>ETGFPEDSEPISISHGNYTKQYPVFVGHKPGRNTTQRHRLDIQMIMIMNGTLYIAARDHIYTVDIDTSHTEEIYCSKKLTWKSRQADVDTCRMKGKHKDECHNFIKVL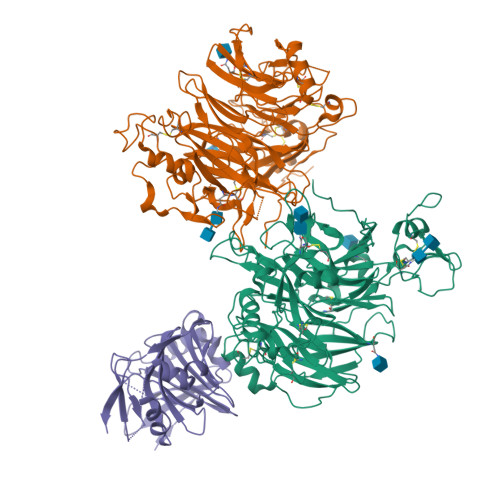LKKNDDALFVCGTNAFNPSCRNYKMDTLEPFGDEFSGMARCPYDAKHANVALFADGKLYSATVTDFLAIDAVIYRSLGESPTLRTVKHDSKWLKEPYFVQAVDYGDYIYFFFREIAVEYNTMGKVVFPRVAQVCKNDMGGSQRVLEKQWTSFLKARLNCSVPGDSHFYFNILQAVTDVIRINGRDVVLATFSTPYNSIPGSAVCAYDMLDIASVFTGRFKEQKSPDSTWTPVPDERVPKPRPGCCAGSSSLERYATSNEFPDDTLNFIKTHPLMDEAVPSIFNRPWFLRTMVRYRLTKIAVDTAAGPYQNHTVVFLGSEKGIILKFLARIGNSGFLNDSLFLEEMSVYNSEKCSYDGVEDKRIMGMQLDRASSSLYVAFSTCVIKVPLGRCERYGKCKKTCIASRDPYCGWIKEGGACSHLSPNSRLTFEQDIERGNTDGLGDCHNGSWSHPQFEK[2x];> SAWSHPQFEKENLYFQGTNVRINLDGNTRSFIVPVITTEQIRKNLSYSFYGSGGSYSLSLSPYNMNIDLNLVENDTWVIDVDNVVKNITIESDEIQKGELIENILSKLNIEDNKIVLNNHTINFYGAINESNRFISLTFSILEDINIIIEIDLVSKSYKILLSGNCIKLIENSSDIQQKIDHIGFNGEHQKYIPYSYIDNETKYNGFIDYSKKEGLFTAEFSNESIIRNIYMPDSNNLFIYSSKDLKDIRIINKGDVKLLIGNYFKDNMKVSLSFTIEDTNTIKLNGVYLDENGVAQILKFMNNAKSALNTSNSLMNFLESINIKNIFYNNLDPNIKFILDTNFIISGSNSIGQFELICDKDKNIQPYFIKFKIKETSYTLYAGNRQNLIVEPSYHLDDSGNISSTVINFSQKYLYGIDRYVNKVIITPNLYTDEINITPVYKPNYICPEVIILDANYINEKINININDLSIRYVWDNDGSDLILIANSEEDNQPQVKIRFVNVFKSDTAADKLSFNFSDKQDVSVSKIISTFSLAAGSENLYFQGHHHHHH>MSKTESYCLEDALNDLFIPETTIETILKRLTIKKNIILQGPPGVGKTFVARRLAYLLTGEKAPQRVNMVQFHQSYSYEDFIQGYRPNGVGFRRKDGIFYNFCQQAKEQPEKKYIFIIDEINRANLSKVFGEVMMLMEHDKRGENWSVPLTYSENDEERFYVPENVYIIGLMNTADRSLAVVDYALRRRFSFIDIEPGFDTPQFRNFLLNKKAEPSFVESLCQKMNELNQEISKEATILGKGFRIGHSYFCCGLEDGTSPDTQWLNEIVMTDIAPLLEEYFFDDPYKQQKWTNKLLGDSSGSHHHHHH[12x];>[2x]MEQPVIPVRNIYYMLTYAWGYLQEIKQANLEAIPGNNLLDILGYVLNKGVLQLSRRGLELDYNPNTEIIPGIKGRIEFAKTIRGFHLNHGKTVSTFDMLNEDTLANRIIKSTLAILIKHEKLNSTIRDEARSLYRKLPGISTLHLTPQHFSYLNGGKNTRYYKFVISVCKFIVNNSIPGQNKGHYRFYDFERNEKEMSLLYQ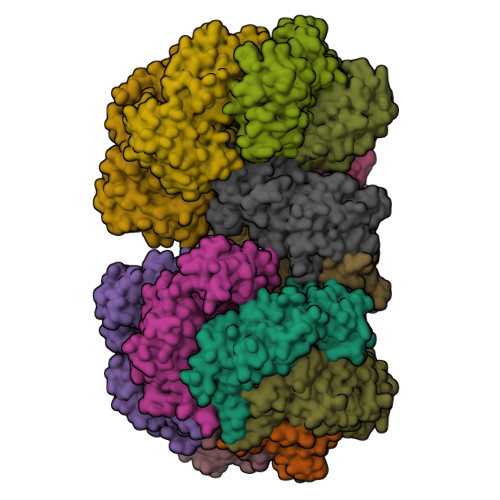KFLYEFCRRELTSANTTRSYLKWDASSISDQSLNLLPRMETDITIRSSEKILIVDAKYYKSIFSRRMGTEKFHSQNLYQLMNYLWSLKPENGENIGGLLIYPHVDTAVKHRYKINGFDIGLCTVNLGQEWPCIHQELLDIFDEYLK> SDPEQLYSTLKNILQQVKNHPNAWPFMEPVKRTEAPGYYEVIRFPMDLKTMSERLRNRYYVSKKLFMADLQRVFTNCKEYNPPESEYYKCASILEK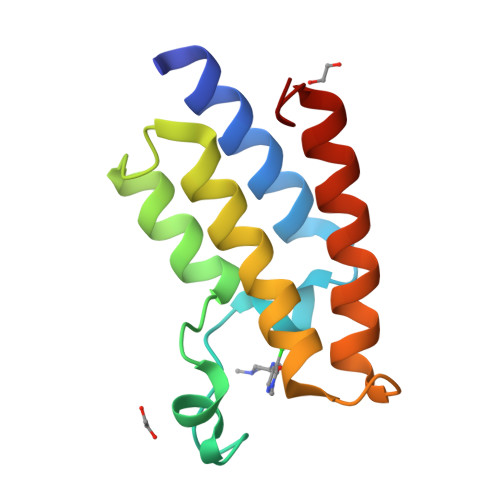FFFSKIKEAGLIDK> MSRRNP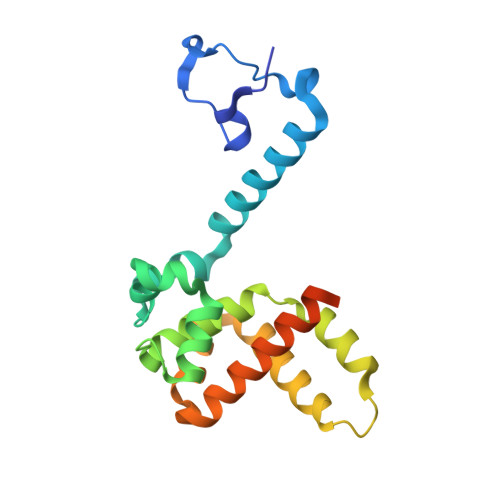CKFEIRGHCLNGKRCHFSHNYFEWPPHALLVRQNFMLNRILKSMDKSIDTLSEISGAAELDRTEEYALGVVGVLESYIGSINNITKQSACVAMSKLLTELNSDDIKKLRDNEELNSPKIRVYNTVISYIESNRKNNKQTIHLLKRLPADVLKKTIKNTLDIHKSITINNPKESTVSDTNDHAKNNDTT>[2x]GPLGSFGQTTPPLVDFLKDILRRYPEGGQMLKELIQNAEDAGATEVKFLYDETQYGTETLWSKDMAPYQGPALYVYNNAVFTPEDWHGIQEIARSRKKDDPLKVGRFGIGFNSVYHITDVPCIFSGDQIGMLDPHQTLFGPHESGQCWNLKDDSKEISELSDQFAPFVGIFGSTKE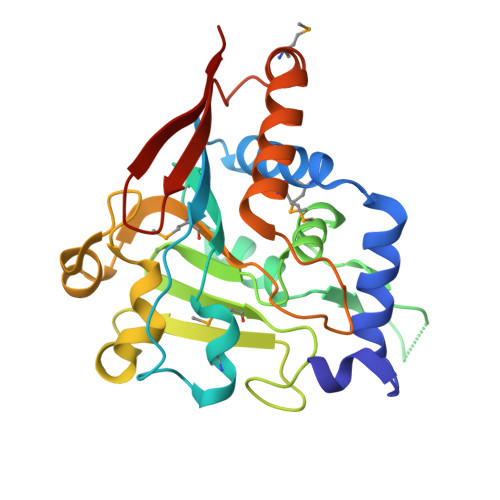TFINGNFPGTMFRFPLRLQPSQLSSNLYNKQMVLELFESFRADADTVLMFLKSVQDVSLYVREADGTEKLVFRVTSS6-CHLORO-N-((3S)-2-OXO-1-{4-[(2S)-2-PYRROLIDINYL]PHENYL}-3-PYRROLIDINYL)-2-NAPHTHALENESULFONAMIDE 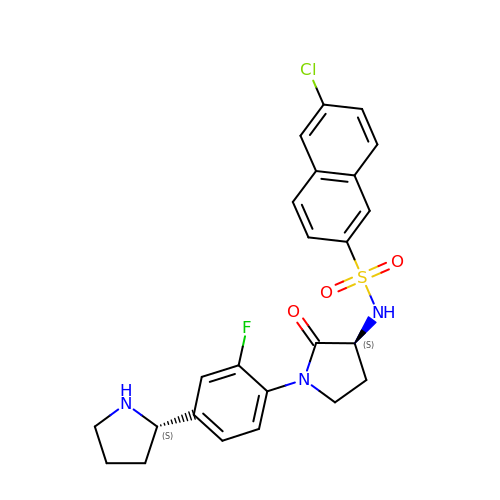| C24 H23 Cl F N3 O3 S | OKMBULRSJZKGQF-VXKWHMMOSA-N> QPIFLNVLEAIEPGVVCAGHDNNQPDSFAALLSSLNELGERQLVHVVKWAKALPGFRNLHVDDQMAVIQYSLMGLMVFAMGWRSFTNVNSAMLYFAPDLVFNEYRMHKSR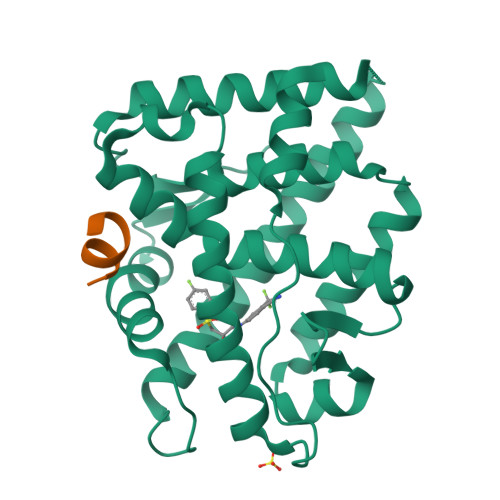MYSQCVRMRHLSQEFGWLQITPQEFLCMKALLLFSIIPVDGLKNQKFFDELRMNYIKELDRIIACKRKNPTSCSRRFYQLTKLLDSVQPIARELHQFTFDLLIKSHMVSVDFPEMMAEIISVQVPKILSGKVKPIYFHTQ;> ANSSFRDWYTSS> MEAAHSKSTEECLAYFGVSETTGLTPDQVKRHLEKYGHNELPAEEGKSLWELVIEQFEDLLVRILLLAACISFVLAWFEEGEETITAFVEPFVILLILIANAIVGVWQERNAENAIEALKEYEPEMGKVYRADRKSVQRIKARDIVPGDIVEVAVGDKVPADIRILSIKSTTLRVDQSILTGESVSVIKHTEPVPDPRAVNQDKKNMLFSGTNIAAGKALGIVATTGVSTEIGKIRDQMAATEQDKTPLQQKLDEFGEQLSKVISLICVAVWLINIGHFNDPVHGGSWIRGAIYYFKIAVALAVAAIPEGLPAVITTCLALGTRRMAKKNAIVRSLPSVETLGCTSVICSDKTGTLTTNQMSVCKMFIIDKVDGDFCSLNEFSITGSTYAPEGEVLKNDKPIRSGQFDGLVELATICALCNDSSLDFNETKGVYEKVGEATETALTTLVEKMNVFNTEVRNLSKVERANACNSVIRQLMKKEFTLEFSRDRKSMSVYCSPAKSSRAAVGNKMFVKGAPEGVIDRCNYVRVGTTRVPMTGPVKEKILSVIKEWGTGRDTLRCLALATRDTPPKREEMVLDDSSRFMEYETDLTFVGVVGMLDPPRKEVMGSIQLCRDAGIRVIMITGDNKGTAIAICRRIGIFGENEEVADRAYTGREFDDLPLAEQREACRRACCFARVEPSHKSKIVEYLQSYDEITAMTGDGVNDAPALKKAEIGIAMGSGTAVAKTASEMVLADDNFSTIVAAVEEGRAIYNNMKQFIRYLISSNVGEVVCIFLTAALGLPEALIPVQLLWVNLVTDGLPATALGFNPPDLDIMDRPPRSPKEPLISGWLFFRYMAIGGYVGAATVGAAAWWFMYAEDGPGVTYHQLTHFMQCTEDHPHFEGLDCEIFEAPEPMTMALSVLVTIEMCNALNSLSENQSLMRMPPWVNIWLLGSICLSMSLHFLILYVDPLPMIFKLKALDLTQWLMVLKISLPVIGLDEILKFIARNYLEG

The fungal H+-ATPase Pma1 belongs to a family of membrane-embedded ATPases that pump ions across cellular membranes, a process energized through transient phosphorylation by ATP. Here we report a compound library screening campaign that identified a series of Pma1 inhibitors that exhibit broad-spectrum antifungal activity. Computer modeling, supported by structural biology indicates that the compounds bind to a groove at the intracellular membrane interface, similar to other P-type ATPase inhibitors that block the ion entry channel. The overall topological organization of all structurally characterized P-type ATPase family members, such as SERCA, the Na+,K+-ATPase, the plant H+-ATPase, the CopA Cu2+-ATPase and the Zn2+-ATPase, is very similar and it is therefore unlikely that the Pma1 structure deviates significantly from its other family members.

To complement the functional data of the tetrahydrocarbazole compounds with structural information, we collected X-ray diffraction data of an inhibitory complex of compound 7 bound to SERCA (rabbit isoform 1a). This complex was formed in a Ca2+-free so-called E2 state and used an ATP analogue, TNPATP, to stabilize the flexible nucleotide-binding region of SERCA, which has been well characterized both functionally and structurally. The 3.0 Å crystal structure of the inhibitory complex shows compound 7 bound at the cytosolic membrane interface, in a groove between transmembrane helices M1, M2, M3 and M4. Despite the modest resolution of 3.0 Å, difference electron density maps clearly allow the placement of bound TNPATP at the ATPase active site, two lipid molecules at the luminal membrane interface (modeled as DOPC), and of compound 7 which is cradled deep inside the cavity marking the cytoplasmic end of the Ca2+ inlet channel of SERCA. However, an anomalous difference map visualizing the isolated signal from the heavy bromine atom in 7 reveals two distinct peaks (5.7 and 7.3 σ) in close vicinity to the tetrahydrocarbazole core. A model with two alternative conformations of the bromo-phenyl moiety, with an occupancy of 0.5 each, allowed a straightforward placement of the bromine atoms into both anomalous peaks. The tetrahydrocarbazole core (modeled with an occupancy of 1) is held in place by three polar contacts to SERCA residues D59 on M1, N101 on M2 and D254 on M3, as well as several hydrophobic interactions involving V62, L65, L98, L253, I307, P312, I315, and the Cβ and Cγ -atoms in the side chain of E309. Interestingly, the SERCA•7•TNPATP complex protein has crystallized in a previously unreported crystal form, reflecting a novel overall conformation of the ATPase. The three cytosolic domains adopt positions roughly halfway in-between the Ca2+-free E2 and the Ca2+-bound E1 state.Members of the aegerolysin protein family are acidic proteins of 13–20 kDa, which are mainly found in bacteria and fungi. In this work, we show for the first time that the bacterial aegerolysin RahU from P. aeruginosa interacts specifically with CPE. The crystal structures of RahU revealed the conserved aegerolysin fold as well as a ligand binding cavity, harbouring a Tris molecule from the crystallization solution. The structures of RahU, in the absence and presence of Tris were determined at 1.27 Å and 1.13 Å resolution, respectively, and reveal a typical aegerolysin fold with a central β-sandwich flanked by a loop containing a short α-helix.

Recombinant RahU protein was expressed using E. coli expression system, purified and subjected to crystallization trials. It is of note that RahU was purified in 20 mM Tris buffer and formed crystals in 0.2 M di-Sodium tartrate, 20% (w/v) PEG 3350. The crystal structure of the apo-RahU was determined at 1.27 Å resolution. The structure shows that RahU is a single domain protein with a distinct β-sandwich architecture that is typical for bacterial and fungal aegerolysins. Furthermore, RahU β-sandwich structure shows structural homology to the superfamily of actinoporins, 20-kDa pore-forming proteins found in sea anemones, with a RMSD value of 2.2 Å when compared to equinatoxin II31 or stycholysin II32. Some of these residues, such as Val20, Ile22, Ile60, Thr72, Phe76, Phe88, Trp90, Asn100 and Trp102, are positioned in the mainly hydrophobic core to maintain the integrity of β-sandwich architecture. However, a majority of the conserved non-alanine and non-glycine residues, including Trp6, Ser16, Asn24, Trp29, Lys31, Lys38, Asp39, Glu41, Ser43, Arg65, Asp77, Asp80, Asp91, Pro93, Trp94, Thr99, Thr101, Ser116, Asn119 and Thr129, is solvent-exposed and/or positioned in the loop areas, possibly providing a uniform environment to aid in the membrane lipid recognition step.

> MAYAEWIAVKVVVSKSIGTVGIRNATLQWGKFYRYTNKDDEISTEEVSSMNVQAGSPQWIASCGRENASSGTQGSFDCYDGNTKMGTFSWDDPWKSGATNTWSFTPASADYAGITSGGNATGTDIGEVTLTLGRFSENLYF> NHSNELPSLCMLNNSFYYMRGGVNTFLIRVSDISVLMKEYDVSIYEPEDLGNCLNKSDSSWAIHWFSNALGHDWLMDPPMLCRNKTKKEGSNIQFNISKADDARVYGKKIRNGMRHLFRGFHDPCEEGKVC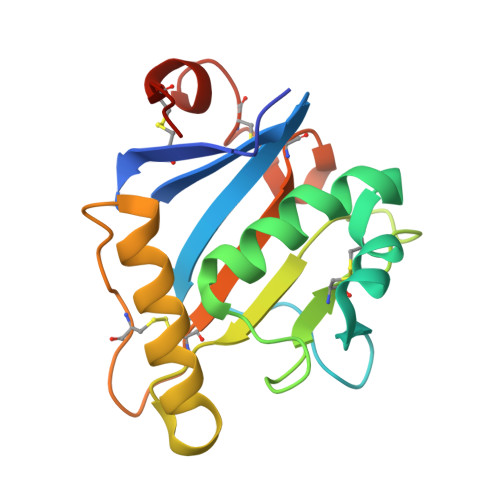YLTINQCGDPSSFDYCGVNHLSKCQFDHVNT A specific SEN biosynthetic pathway was identified in Variovorax paradoxus DSM 30034, which is recognized as a way to incorporate Se into organic matter in bacteria. The bacterial SEN biosynthesis gene cluster encodes three proteins, SenA, SenB, and SenC. SenB catalyzes the generation of the key intermediate selenoglucose product using SeP synthesized by selenophosphate synthetase (named SelD or SenC)15. In contrast to other types of GTs, SenB performs dual functions in two-step catalytic reactions, catalyzing the formation of C–Se glycosidic bonds and the subsequent cleavage of Se-P bonds to generate the final product.

We selected two SenB-like enzymes, CbSenB (GenBank: RYF17368.1; 65.5% sequence similarity), which was derived from Comamonadaceae bacterium, and RsSenB (GenBank: MBC7468551.1, 65.2% sequence similarity), which was derived from Ramlibacter sp., for further functional characterization. Like SenB, CbSenB and RsSenB are located in the SEN biosynthesis-related gene cluster. Catalytic activity analysis revealed that CbSenB and RsSenB recognize sugar donors like SenB and utilize UDP-Glc, UDP-GlcNAc, UDP-Gal, and UDP-GalNAc to generate the corresponding selenosugars. The catalytic activities of these three enzymes for UDP-Glc, UDP-GlcNAc, and UDP-Gal were similar, but RsSenB utilized UDP-GalNAc more strongly than SenB and CbSenB did. Mutagenesis assays confirmed that the residues equivalent to N20/T23/E231 of SenB are critical for acceptance of various sugar donors in CbSenB and RsSenB. Unlike that of SenB, the asymmetric unit of the crystal contains two RsSenB molecules. The monomer structure of RsSenB is very similar to that of SenB, with an RMSD of 0.99 Å for Cα atoms. The spatial positions of the putative catalytic residue K158 in RsSenB strongly overlapped with the structures of SenB. In addition, the mutagenesis results for the catalytic residues in CbSenB and RsSenB were consistent with those for SenB. These results not only provided two other SeGTs but also further demonstrated the universal effects of the key amino acids N20/T23/E231 on the promiscuity of sugar donors and the putative catalytic residue K158 on the Se glycosylation of SenB.

>MSRPSVAIVSPAVASANNGNWQTARRWQEFLDGTCNVRMTQRWPDDGSQDDVVMLALHARRSADSIEAWASVHGDRGLAVVLTGTDLYQDIVVDPRARHSLELAGQLVVLQDLGAEALPPALRGKTRVIYQSTPSQAAASKPDTVLQALMVGHLREVKSPQTLFQAARLLAGHDDIRIDHIGEALDPVLGEQALATQRDCPNYRWLGALPHDGTRERIRCAHLLVHASAMEGGAHVIMEAVCSGTPVLASRIPGNVGMLGADYAGYFTHGDAAALAALLVRCRQGQAASGDVPADPLLARLGAQCALRAPLFAPEAERAALLRLVADLM[2x]> MGSSHHHHHHSQDPMDIKINGIKKYTIHVLAKVSASGMEFTQEKDFEHQLLLTDMLETVIRKSVEVNPVLHFHLRKSIIMNHSYFILGLNYIPPAFATKNVKSIHEIYQAIQDVNDLQLLDEFEKSKEKLINKIQQYKHSDSHSGSIRLKDRLFADKKYGSDRLGNFEKMNKITDNIIYAAPDMVNKICEGDGLFYHINDGAIHISNIKDFNYYIPAVINEGVEDIRTDFSKEYSILTCAYTFEHVTDLEREILIPMFDGYIGKYGHSVLFKTLRLVDENLYHISSHYDQESNLLFITVLCSKNQLSTILTKIQHTIESIEFDSVSFSLSKVMFENESRFRFEDINGLLSHVIKQHGEYKNPESFLKAIQNTDIADFYRLKANMRWVGTSIVEGG;> MLNKSFVKKLDESLNRKQVGSTNVTRYKIEDSYLVLAAVRVGIGGLTYHNGAAAFLEALKFWRYGENIYNLFFQRGAILNAYTTLEFTDYVFLSKEESINENLNLLLTFLYHHQYDEKTISLERNIIINEINGAGTARLNGQESIEKERHCILGSAESISRMGRKEFELISQKYYTPENTSIYVIGGNQDIDLFHIPTAVMTTQYGKPTHKVNVNEVEMNKDMILLPVEHGDYLKNRMICHLIADMIKHLAQQLE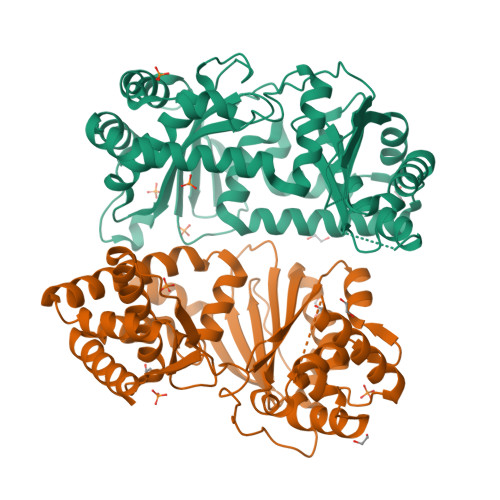YDVSVGLFISTNQHSCYLKVKKSDQKRFSSLIQQLSMDEHFIETYIKDYQWRFMNELVINFNQLHNIYDYMTEYRLGEYTVAELFGSLDSVDKLDILAVRNELINQLTVGE>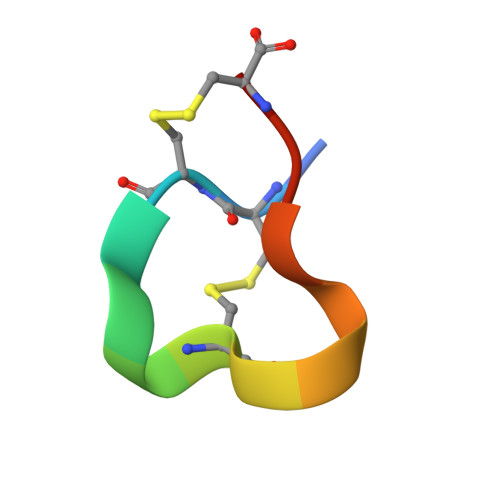 ICCNPACGPKYSCX> STLRLRGDLPERVDLLNITPLALSGLSETEAGKLAIGTSRRGLTLGDVFEIRLDGSDSLVIEGGSARLDRVGAALSQGSIRVEGDVGQRLGEGMAAGTLTVTGSAGPYAGTGATGGTITIEGDAGDHAGGAVYAAKAGLDGAT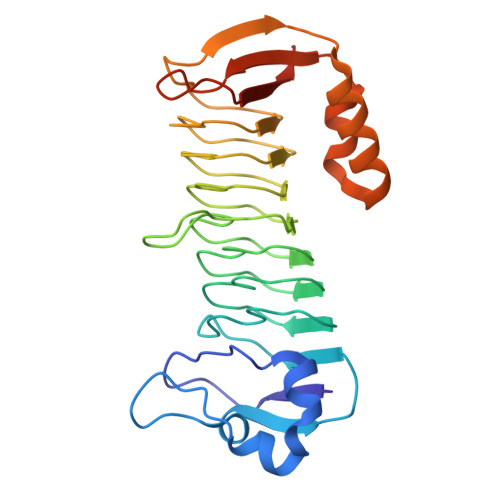LVIKGAAGDHLGDRMRRGMILAGSAGAFAASRMIAGTIVVSGALGDHPGYGMRRGTLIAGSHGTLLPTFVETGTPDLVFVRLLAQSLKHLGAAQANLLSGTLRRYSGDLATLGKGELFVPAHGSAWSHPQFEK> MPRPGHIAMVSVPSRGHLHPSLELIRELVARGHRVTYANDPSVAAAVTETGAELVPYTSALPSTDTTEGRVTDQIAQMDVFLDDAVGMLPQLRAAYEEDRPDVFLYDVLAYPARVLAMNWGIPSIQISPTWVMPEKYRERMAPVVEQLKQDPRGAAHYRRFDAWLEDSGVPGIDAGDLVNLPERSLVLVPRFLQPDADDVDEKRFTFIGPCLGRRAHQGDWKRPAGAEKVALVSLGSHLTNQLPFYETCVEVFAALPDWHLVLQIGRHVDAGELGELPPNVEVHNWVPQLAVLEQADVFVTHGGMGGIQEGLFSGVPMVVAPQANDQPANAESV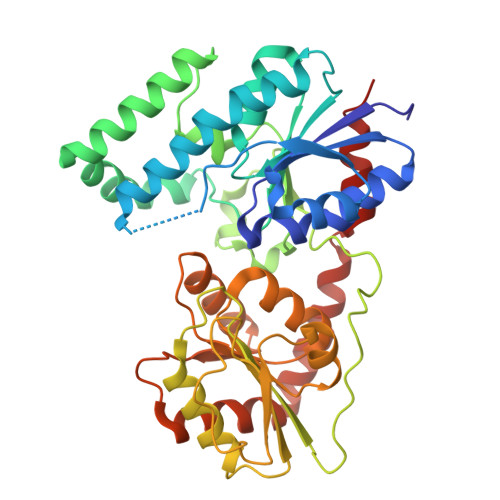VGLGIARRIDIATVTPDRLRAAVVELASDPAVAERLSGLRRELRAHGGTMRAADLIERQLPA>[4x]SMGEIESYCNKELGPLPTKAPTLSKNVLDLFSLKGKVASVTGSSGGIGWAVAEAYAQAGADVAIWYNSHPADEK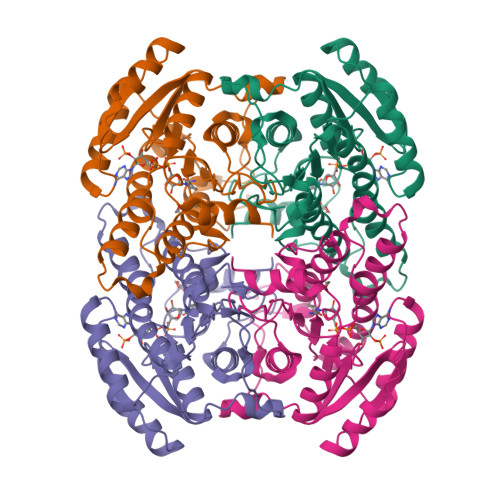AEHLQKTYGVHSKAYKCNISDPKSVEETISQQEKDFGTIDVFVANAGVTWTQGPEIDVDNYDSWNKIISVDLNGVYYCSHNIGKIFKKNGKGSLIITSSISGKIVNIPQLQAPYNTAKAACTHLAKSLAIEWAPFARVNTISPGYIDTDITDFASKDMKAKWWQLTPLGREGLTQELVGGYLYLASNASTFTTGSDVVIDGGYTCP> EGPTFQDVASQVFGQAVGPDNDGTLYVFGLTAKYTKPDYVDGRGPYKSFLKFLPSIRWYDPEHYWTNGSQNEGVFKNEECVLCHTVQTPTIVKDWKKSAHGNLE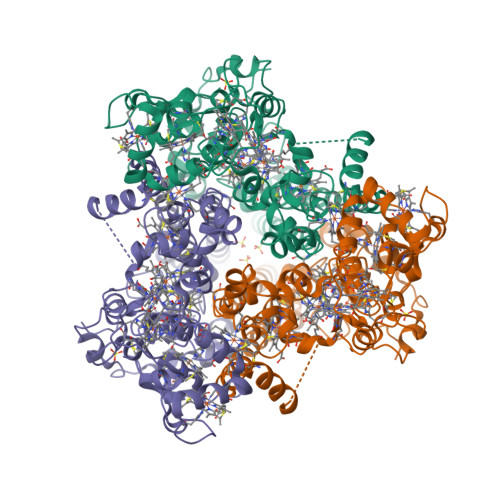MRRGLGVKGKDGKPVEGTVGCDACHGNDHQKLFMPTYKNCGECHPRETSEHRSGGLGSHTHAYTVNVLEFSWHVGKPAEEVAGCAECHAIVENRCDGCHTRHVFSPAEARKPTACRYCHMGIDHDEWAMYNTSVHGCLYEAESATMDWSKPSKKGNYRVPTCAYCHMQDGNHNPQQFGTIYSDMGMFQVDRGAPKHKAKRDAWIKKCQDCHSPRFAADKLKEMDAGVNLSFTKWREAAAVIVGCFLDGVVDPMPEGSPPDWYGHYTFSLLPGGDPRFYATSNLERLGLEMICYLTGNVYKAYAHMSMYNQTYGNGSAFEQDRKLVEIKTEAAKLRRFAAIEKKIGLEHKSEGFWQHGEYLDLLPGWIRKPGDVDVEWFKRTDIPHRANADAGVAPHGH> DSKLSIISWNVDGLDTLNLADRARGLC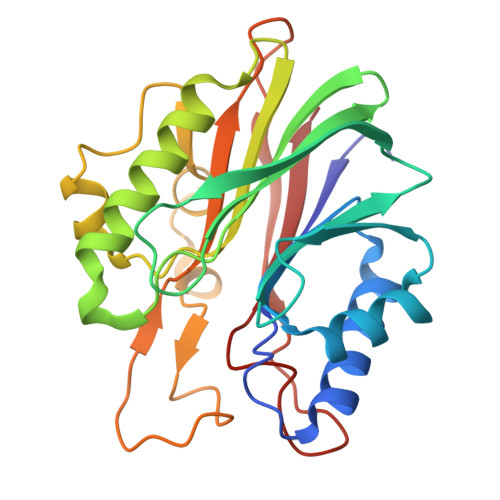SYLALYTPDVVFLQELIPAYVQYLKKRAVSYLFFEGSDDGYFTGIMLRKSRVKFLESEIICFPTTQMMRNLLIAQVTFSGQKLYLMTSHLESCKNQSQERTKQLRVVLQKIKEAPEDAIVIFAGDTNLRDAEVANVGGLPAGVCDVWEQLGKQEHCRYTWDTKANSNKTVPYVSRCRFDRIFLRSAKTAPPVTPDHMALIGMEKLDCGRYTSDHWGIYCTFNT>MAGPVDNIKPMKYNDPANGVESSIGPQIHTRYWYKRALIDAAKEAYFGQLADTFSMPKHYGKEIVRLHYIPLLDDRNVNDQGIDASGATIANGNLYGSSRDVGNITAKMPTLTEIGGRVNRVGFKRVEIKGKLEKYGFFREYTQEQLDFDSDPAMEGHVTTEMVKGANEITEDLLQIDLLNSAGTVRYPGAATSDAEVDASTEVTYDSLMRLRLDLDNARAPTKIKMITGTRMIDTRTVGNARALYVGSDLVPTIEAMKDNHGNPAFIPIEKYAAGGATMHGEVGQLGRFRVIVNP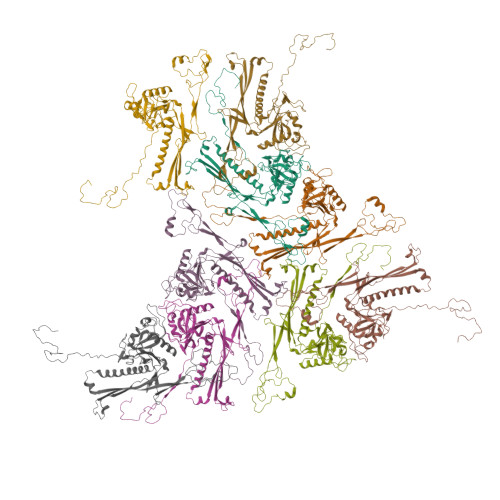QMMHWAGVGKAVDPNDQVPMHESGGKYSVFPMLCVASEAFTTVGFATDGKNVKFKIITKRPGEATADRSDPYGEMGFMSIKWYYGFMVFRPEWIALLKTVARL[9x]>GSRSGVAVADESLTAFNDLKLGKKYKFILFGLNDAKTEIVVKETSTDPSYDAFLEKLPENDCLYAIYDFEYEINGNEGKRSKIVFFTWSPDTAPVRSKMVYASSKDALRRALNGVSTDVQGTDFSEVSYDSVLEDVSR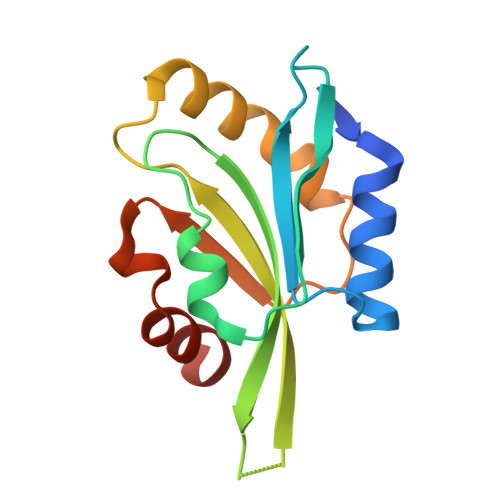GAGSH[2x]>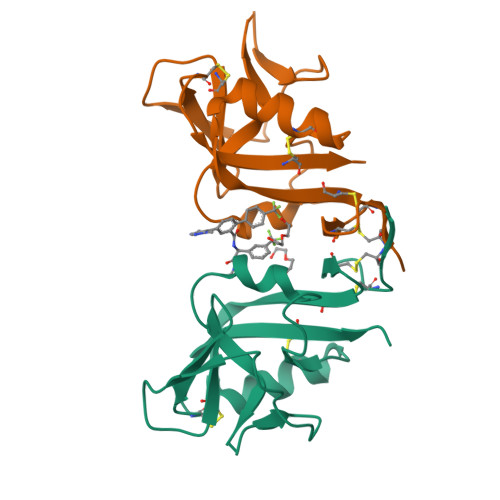[2x]MGPLTESYCGPCPKNWICYKNNCYQFFDEEKNWYESQASCMSQNASLLKVYSKEDQDLLKLVKSYHWMGLVHIPTNGSWQWEDGSSLSPNLLTIIEMQKGDCALYASSFKGYIENCSTPNTYICMQRTV>SLGSDADSAGSLIQPMQIPGIIMPGLRRLTIRDLLAQGRTSSNALEYVREEVFTNAPGDSDITFSKQTANVKTIAHWVQASRQVMDDAPMLQSYINNRLMYGLALKEEGQLLNGDGTGDNLEGLNKVATAYDTS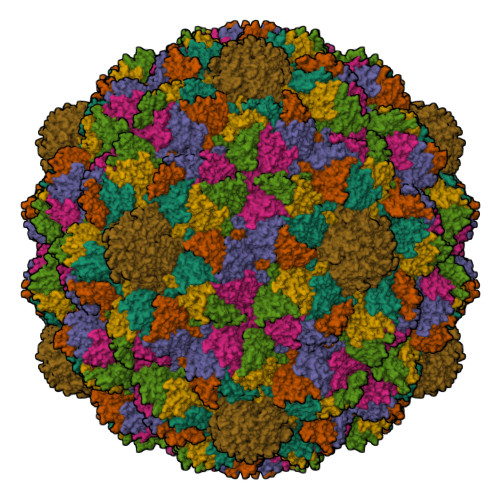LNATGDTRADIIAHAIYQVTESEFSASGIVLNPRDWHNIALLKDNEGRYIFGGPQAFTSNIMWGLPVVPTKAQAAGTFTVGGFDMASQVFDRMDATVEVSREDRDNFVKNMLTILCEERLALAHYRPTAIIKGTFSSGS[7x]>[2x]MANPYERGPNPTDALLEARSGPFSVSEERASRFGADGFGGGTIYYPRENNTYG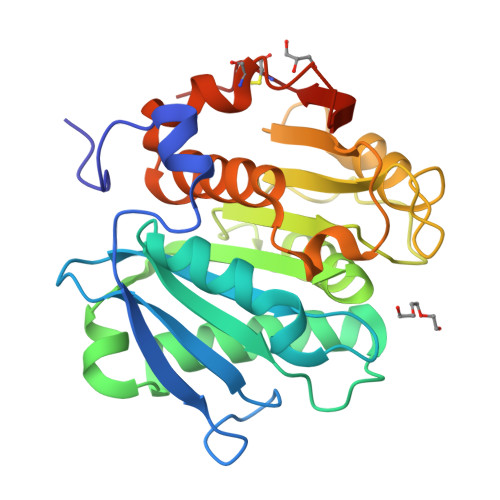AVAISPGYTGTQASVAWLGERIASHGFVVITIDTNTTLDQPDSRARQLNAALDYMINDASSAVRSRIDSSRLAVMGHSMGGGGTLRLASQRPDLKAAIPLTPWHLNKNWSSVRVPTLIIGADLDTIAPVLTHARPFYNSLPTSISKAYLELDGATHFAPNIPNKIIGKYSVAWLKRFVDNDTRYTQFLCPGPRDGLFGEVEEYRSTCPFLEHHHHHH>[2x]MGHHHHHHHHHHSSGHIDDDDKHMCGNSIDEKTVKKYENQLNQTVKQEIASLSQDSGIKIEFSDFKCNADGDFIA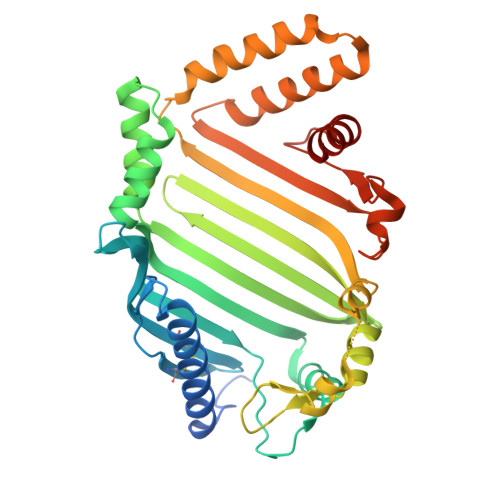CLSPNFKTLAKDNNDEYQELFQAKNIKIRSNEIYKGETNTSISIKEYYNDLFKNQKSIQSNLVFEDFKLGEKVVSDINASLFQQDPKISSFINKLSSDSYTLSFDNSINKQENNYLDNLDIKFYNAKLNFNTNLNINLKEDLLNYLDSKGIKFNTQTLAMDEQAINELLNMVNYEQASDFSNTIQKYIILNNFKIDSTLKTEGVFSSYIATAKENLQTLKAQSQNEEQALIFDKALAILNNITQNDDYKLNLDLKFKNIPVSDYSTQGIDSIEKLSINNQDATEALKIILPFIMFSMLMGGASF>[3x]GSSGSSGMTQLALIGLWIGFIGMVIGAVIFGQKAVAMRRKEGMEFPLKSFFIVLWAGALYLTMILGETVTPVKDQTVFWGRYVDWVVTTPVLLLDLGVLAGLRPKLIAGVIAADIFMILTGLVATLEAPPTSYLWYIISCGAFIAILASLLTEFTASAARRNVRVNNLFLKLRNYLIVLWICYPIVWLLGAEAFKIIPTGVEVVIYAIIDIAAKVGFGLILTSAAPEILAQASNSESFMEAVHSYMGKGERERDRSYTP

Rhodopsins are seven-transmembrane proteins that contain retinal as a light-absorbing chromophore and a light-induced trans–cis isomerization of retinal triggers their activities. There are, however, 9 genomes from a high salinity environment, 8 were from the same site and showed little genetic variation. Phylogenetic analysis of the amino acid sequences of the rhodopsins encoded by the 56 identified genes revealed that the proteins belonged to four known rhodopsin clades: XLR (3 genes), NaR (1 gene), XeR (15 genes), and CyHR (24 genes) and one novel clade (13 genes); the novel rhodopsin clade consisted entirely of rhodopsin genes from cyanobacterial genomes so we named the clade “cyanorhodopsin” (CyR). All of the CyRs included Lys204N2098R in the seventh helix (helix G), which is known to make a Schiff base linkage between the rhodopsin protein moiety and the retinal chromophore in other rhodopsins. Heterologous rhodopsin gene expression analysis showed that the rhodopsins in the CyR clade function as light-driven outward H+ pumps.

The crystal structures of cell-free-synthesized N2098R and N4075R were determined at 2.65 Å and 1.9 Å resolution, respectively. Since the two structures were almost identical, only the structure of N2098R is described. Next, to further examine the ion-transporting activities of the CyRs, we heterologously expressed three synthesized rhodopsin genes—N2098R (BAY09002.1), B1401R (WP_074382570.1), and N4075R (GAX43141.1)—in Escherichia coli. A light-induced decrease in pH was observed in the suspensions of the cells expressing each of the rhodopsins (solid line), and this decrease was almost completely abolished in the presence of the protonophore carbonyl cyanide m-chlorophenylhydrazone (CCCP) (broken line). These results showed that N2098R and B1401R transport proton from the cytoplasmic side to the extracellular space. On the other hand, N4075R was thought to act as an outward proton pump, but its activity was smaller than that of the others. Therefore, the possibility of transporting other ions cannot be excluded.>[2x]GIKGIYKEIGSGERISLCKLAIDHLE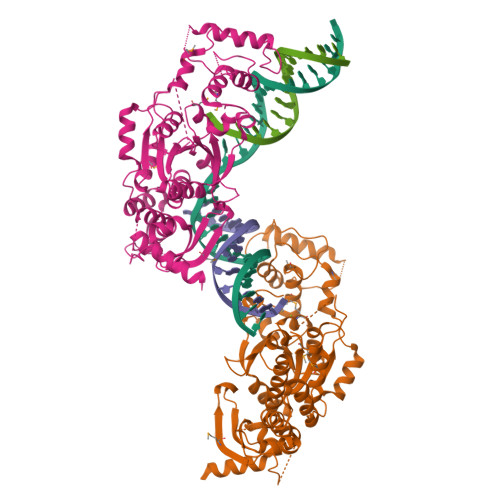QHNRPLRLAIDMAIWQFQIQAARGGSNPAIRTLFYRFVRLLSLGIHPIFVFDGPNKPIFKRNRRSGTGNGVSTAMAKRLIRLFGFTAHDAPGEAEAECAYLEQQGIVDAVLSEDVDTIMFGSRVTLRDWSSEGSKGGPPTHVTLHDAKKIAEGPSGLDREGMVLVALMSGGDYLPDGIPGCGIKVACQAAKAGFGKELCRIKRADKEAITEWKQRLLHELRTNESGFFRTKHKALEIPENFPNMEVLRYYTHPVVSSPATIERLRQEFPPSSTVDIAGLREFTRETFDWTFRPGAIKLIKVLAPGLLVQRCLDRYVSGPRIDDPDLKKKEESTLVKGISMRREHFSTDATPELRVSFIPAELVGLDPGQEPEVQVEAFGRSGLALNSDDEFDEDISSSQKAPKKPFDPWQPDLAWVPETILKLGVPVTVEDWEEGQRS> ATLDSWLSNEATVARTAILNNIGADGAWVSGADSGIVVASPSTDNPDYFYTWTRDSGLVLKTLVDLFRNGDTSLLSTIENYISAQAIVQGISNPSGDLSSGAGLGEPKFNVDETAYTGSWGRPQRDGPALRATAMIGFGQWLLDNGYTSTATDIVWPLVRNDLSYVAQYWNQTGYDLWEEVNGSSFFTIAVQHRALVEGSAFATAVGSSCSWCDSQAPEILCYLQSFWTGSFILANFDSSRSGKDANTLLGSIHTFDPEAACDDSTFQPCSPRALANH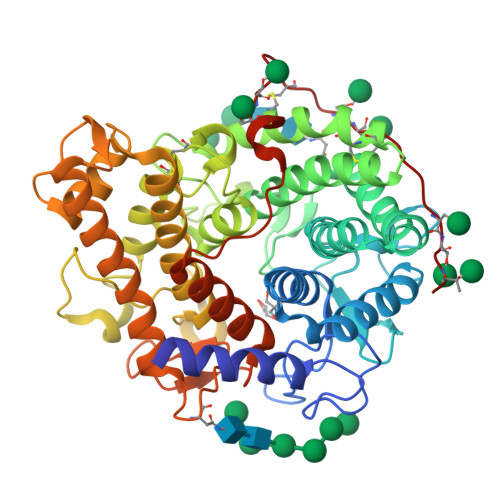KEVVDSFRSIYTLNDGLSDSEAVAVGRYPEDTYYNGNPWFLCTLAAAEQLYDALYQWDKQGSLEVTDVSLDFFKALYSDAATGTYSSSSSTYSSIVDAVKTFADGFVSIVETHAASNGSMSEQYDKSDGEQLSARDLTWSYAALLTANNRRNSVVPASWGETSASSVPGTCAATSAIGTYSSVTVTSWPSIV> SIVTKSIVNADAEARYLSPGELDRIKSFVTSGERRVRIAETMTGARERIIKQAGDQLFGKRPDVVSPGGNAYGADMTATCLRDLDYYLRLITYGIVAGDVTPIEEIGVVGVREMYKSLGTPIEAIAEGVRAMKSVATSLLSGADAAEAGSYF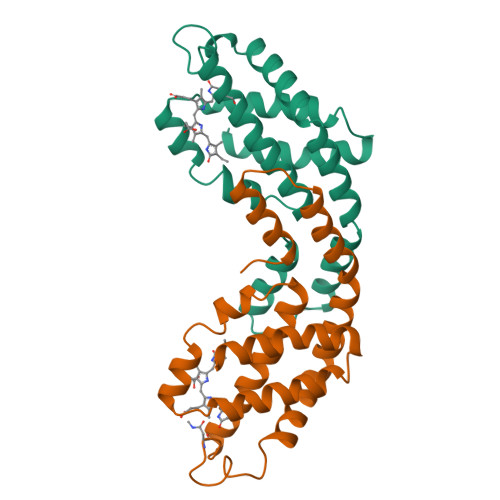DYLIGAMS;> MQDAITSVINSSDVQGKYLDASAIQKLKAYFATGELRVRAATTISANAANIVKEAVAKSLLYSDVTRPGGNMYTTRRYAACIRDLDYYLRYATYAMLAGDPSILDERVLNGLKETYNSLGVPIGATVQAIQAMKEVTAGLVGGGAGKEMGIYFDYICSGLS4-Cl-Bn7GpppG mRNA 5' cap analog | C27 H33 Cl N10 O18 P3 | 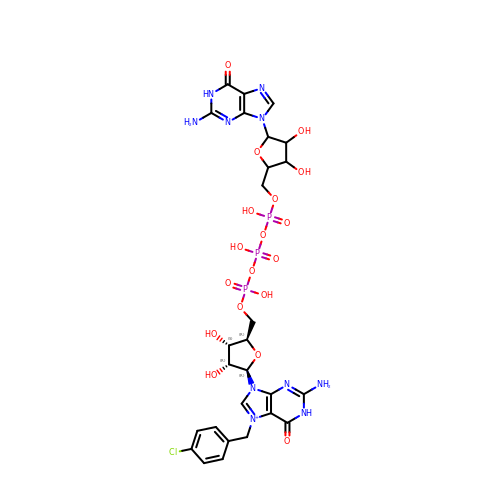YLIRYFJCSIVXAE-AGNUKMHHSA-O N-[(2S)-3-[(S)-(4-bromophenyl)(hydroxy)phosphoryl]-2-{[3-(3'-chlorobiphenyl-4-yl)-1,2-oxazol-5-yl]methyl}propanoyl]-L-alpha-glutamyl-L-alpha-glutamine | C35 H35 Br Cl N4 O10 P | 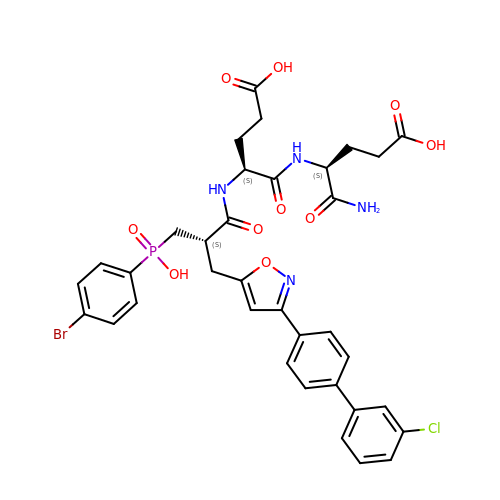PTUCPHGSAFOJAU-MGONOCMRSA-N> HNMKAFLDELKAENIKKFLYNFTQIPHLAGTEQNFQLAKQIQSQWKEFGLDSVELAHYDVLLSYPNKTHPNYISIINEDGNEIFNTSLFEPPPPGYENVSDIVPPFSAFSPQGMPEGDLVYVNYARTEDFFKLERDMKINCSGKIVIARYGKVFRGNKVKNAQLAGAKGVILYSDPADYFAPGVKSYPDGWNLPGGGVQRGNILNLNGAGDPLTPGYPANEYAYRRGIAEAVGLPSIPVHPIGYYDAQKLLEKMGGSAPPDSSWRGSLKVPYNVGPGFTGNFSTQKVKMHIHSTNEVTRIYNVIGTLRGAVEPDRYVILGGHRDSWVFGGIDPQSGAAVVHEIVRSFGTLKKEGWRPRRTILFASWDAEEFGLLG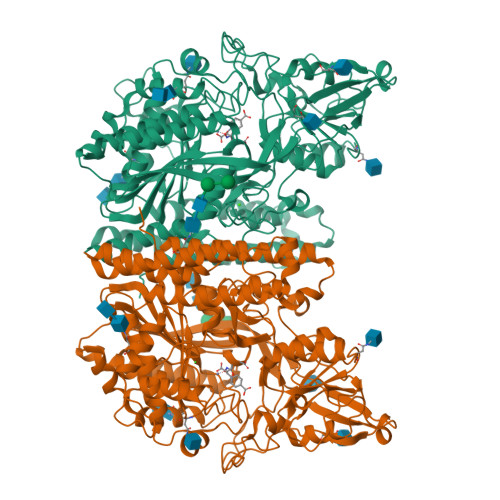STEWAEENSRLLQERGVAYINADSSIEGNYTLRVDCTPLMYSLVHNLTKELKSPDEGFEGKSLYESWTKKSPSPEFSGMPRISKLGSGNDFEVFFQRLGIASGRARYTKNWETNKFSGYPLYHSVYETYELVEKFYDPMFKYHLTVAQVRGGMVFELANSIVLPFDCRDYAVVLRKYADKIYSISMKHPQEMKTYSVSFDSLFSAVKNFTEIASKFSERLQDFDKSNPIVLRMMNDQLMFLERAFIDPLGLPDRPFYRHVIYAPSSHNKYAGESFPGIYDALFDIESKVDPSKAWGEVKRQIYVAAFTVQAAAETLSEVA> GPVGEPVASEINEASKVSSRLLTQDILFRKDRQATISLPIKLPVEDIITQTCDKITYGPLKFLDLLEKETA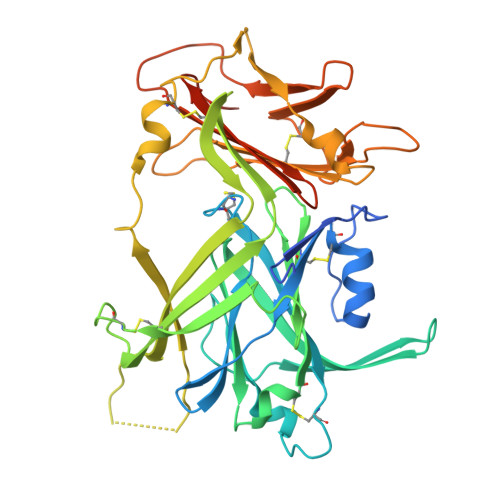VLPLSTDITCPACLGRAVLVGKWECPAHVAVNESDLTVFGPNKEEHVPQFVTVQQPSDGKMQRLFFAKFLGTEESLAVLRVPGPDGHLCIQEALIHFKELSGAGVCSLWKANDSREEGLEMKQVDCLETTVLENQTCIATTLSKKIYHRLYCGERLMTGGQVSTRVLLTALGFYKRQPYTFHRVPKGMVYVHLIDSGSEDYMEYSECEEVTPGRYEDKQISYTFYTDLFQTADGEPVLASVWGTSGLKDSAYESCAFVIPTDGEEDLVPRRIMSKCYPFRLTYHPSTMTVRLDVRVEKHHGATDQGFVFLKMESGTYSEGREYYLDRVLWGEDSSTNNVLQHHHHHHHH>GNYKKPKLLYCSNGGHFLRILPDGTVDGTRDRSDQHIQLQLSAESVGEVYIKSTETGQYLAMDTDGLLYGSQTPNEECLFLERLEENHYNTYISKKHAEKNWFVGLKKNGSCKRGPRTHYGQKAILFLP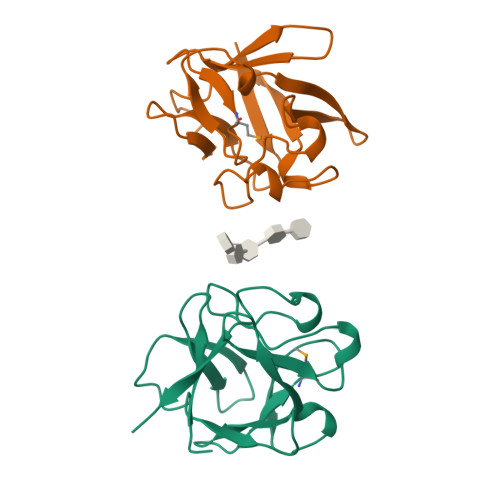LPVSSD[6x]> MSLADTVRMGTEGAYPPYNFINDAGEVDGFERELGDELCKRAGLTCEWVKNDWDSIIPNLVSGNYDTIIAGMSITDER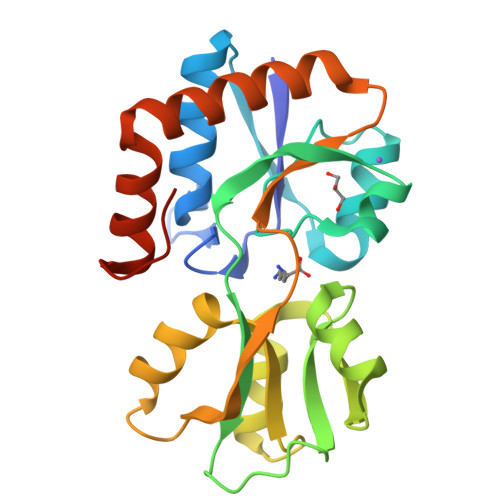DEVIDFTQNYIPPTASSYVATSDGADLSGIVAAQTATIQAGYIAESGATLVEFATPEETIAAVRNGEADAVFADRDYLVPIVAESGGELMFVGDDVPLGGGVGMGLRESDGELRGKFDAAITSMKEDGTLNTMIKKWFGEDAAVYEEGHHHHHH> KKAVPYNRMKLMIVGNTGSGKTTLLQQLMKTKKSDLGMQSATVGIDVKDWPIQIRDKRKRDLVLNVWDFAGREEFYSTHPHFMTQRALYLAVYDLSKGQAEVDAMKPWLFNIKARASSSPVILVGTHLDVSDEKQRKACMSKITKELLNKRGFPAIRDYHFVNATEESDALAKLRKTIINESLNFKIRDQLVVGQLIPDCYVELEKIILSERKNVPIEFPVIDRKRLLQLVRENQLQLDENELPHAVHFLNESGVLLHFQDPALQLSDLYFVEPKWLCKIMAQILTVKVEGCPKHPKGIISRRDVEKFLSKKRKFPKNYMTQYFKLLEKFQIALPIGEEYLLVPSSLSDHRPVIELPHCENSEIIIRLYEMPYFPMGFWSRLINRLLEISPYMLSGRERALRPNRRYWRQGIYLNWSPEAYCLVGSEVLDNHPESFLKITVPSCRKGCILLGQVVDHIDSLMEEWFPGLLEIDICGEGETLLKKWALYSFNDGEEHQKILLDDLMKKAEEGDLLVNPDQPRLTIPISQIAPDLILADLPRNIMLNNDELEFEQAPEFLLGDGSFGSVYRAAYEGEEVAVKIFNKHTSLRLLRQELVVLCHLHHPSLISLLAAGIRPRMLVMELASKGSLDRLLQQDKASLTRTLQHRIALHVADGLRYLHSAMIIYRDLKPHNVLLFTLYPNAAIIAKIADYGIAQYCCRMGIKTSEGTPGFRAPEVARGNVIYNQQADVYSFGLLLYDILTTGGRIVEGLKFPNEFDELEIQGKLPDPVKEYGCAPWPMVEKLIKQCLKENPQERPTSAQVFDILNSAELVCLTRRILLPKNVIVECMVATHHNSRNASIWLGCGHTDRGQLSFLDLNTEGYTSEEVADSRILCLALVHLPVEKESWIVSGTQSGTLLVINTEDGKKRHTLEKMTDSVTCLYCNSFSKQSKQKNFLLVGTADGKLAIFEDKTVKLKGAAPLKILNIGNVSTPLMCLSESTNSTERNVMWGGCGTKIFSFSNDFTIQKLIETRTSQLFSYAAFSDSNIITVVVDTALYIAKQNSPVVEVWDKKTEKLCGLIDCVHFLREVTVKENKESKHKMSYSGRVKTLCLQKNTALWIGTGGGHILLLDLSTRRLIRVIYNFCNSVRVMMTAQLGSLKNVMLVLGYNRKNTEGTQKQKEIQSCLTVWDINLPHEVQNLEKHIEVRKELAEKMRRTSVE

Leucine-rich repeat kinase 2 (LRRK2) is a highly pursued drug target for Parkinson’s disease (PD), which is the second most common neurodegenerative disease projected to affect 17.5 million people by 20401. LRRK2 is a 286-kDa protein containing seven domains (ARM, ANK, LRR, ROC, COR, KIN, and WD40) with kinase and GTPase activities. Autosomal dominant LRRK2 mutations with higher kinase activity are leading genetic causes of both familial and sporadic late-onset PD cases. Here we report high-resolution cryo-EM structures of LRRK2 in complex with a panel of small molecules, including two type I (LRRK2-IN-1 and GNE-7915) and three type II inhibitors (rebastinib, ponatinib, and GZD-824).

For type I inhibitors, we designed an LRRK2RCKW construct with M1732R mutation (LRRK2RCKWm) based on the following observations and rationales. Therefore, we introduced the M1732R mutation, which disrupts COR-B dimerization and LRRK2 filamentation, to prevent protein aggregation. Second, the binding of type I inhibitors could lead to a kinase-closed active-like conformation with flexible N-terminal ARM-ANK-LRR domains, which did not show interaction with the rest of the protein upon activation. We determined LRRK2RCKWm structures with LRRK2-IN-1 and GNE-7915 at overall resolutions of 3.5 and 3.8 Å, respectively. Despite small differences in the overall structures, LRRK2 KIN domains with type I inhibitors and ATP are almost identical with RMSD < 0.5 Å. LRRK2-IN-1 has an IC50 of 65.1 nM to LRRK2 and 1.27 mM to Roco4. Phe1107 and Phe1161 correspond to Leu1949 and Leu2001 in LRRK2, and side chains of both residues in LRRK2 point towards and interact with LRRK2-IN-1. Furthermore, the 1-methylpiperazine group of LRRK2-IN-1 makes more intensive interactions with the kinase N lobe of LRRK2, forming a more intensive and complementary interaction interface, which could, at least partially, contribute to another two orders of magnitude of IC50 difference between LRRK2 and Roco4 with F1107L and F1161L mutations. The cavity shaped by KIN and COR domains in the active-like LRRK2–LRRK2-IN-1 complex is sealed by KIN–COR interactions. This is accompanied with the opening of COR-A and COR-B subdomains, more intensive interactions between the KIN N lobe and COR-B, and a novel interface between the KIN C lobe and COR domain.>[8x]TPEEAQREKDTRISKKMETMGIYFATPEWVALNGHRGPSPGQLKYWQNTREIPDPNEDYLDYVHAEKSRLASEEQILRAATSIYGAPGQA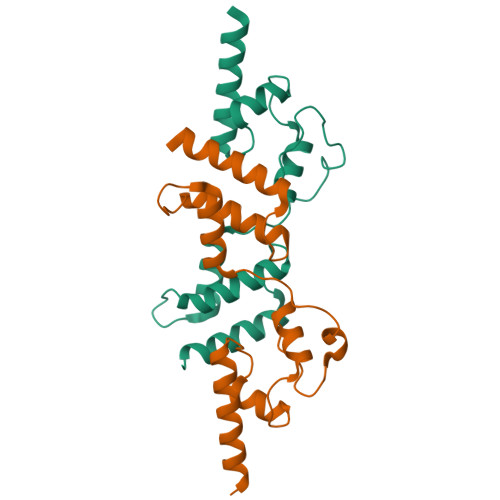EPPQAFIDEVAKVYEINHGRGPNQEQMKDLLLTAMEMKHRN>[18x]MTAVSEFRPGLEGVPATLSSISFVDGQRGVLEYRGISIEQLAQQSSFLETAYLLIWGHLPTQQELTEFEHEIRYHRRIKFRIRDMMKCFPDSGHPMDALQASAAALGLFYSRRALDDPEYIRAAVVRLLAKIPTMVAAFQLIRKGNDPIQPRDELDYAANFLYMLTEREPDPVAARIFDICLTLHAEHTINASTFSAMVTASTLTDPYAVVASAVGTLAGPLHGGANEEVLDMLEAIGSVENVEPYLDHCIATKTRIMGFGHRVYKVKDPRAVILQNLAEQLFDIFGHDPYYEIAVAVEKAAAERLSHKGIYPNVDFYSGLVYRKLGIPSDLFTPVFAIARVAGWLAHWKEQLNENRIFRPTQIYTGSHNLDYTPIADRDLAIESDLEHHHHHH

Here we report the discovery of a natural protein, citrate synthase from the cyanobacterium Synechococcus elongatus, which self-assembles into Sierpiński triangles. Bacterial citrate synthase (CS) proteins are homo-oligomeric enzymes that can assemble into dimers and hexamers. CS catalyses the condensation of acetyl-CoA and oxaloacetate to citrate as the first step in the tricarboxylic acid cycle. Using cryo-electron microscopy, we reveal how the fractal assembles from a hexameric building block.

Three dimers are first arranged in a hexameric ring and three hexamers then connect into a triangle. In the 18mer (level 1), CS dimers assemble into hexamers through a heterologous interface similar to known hexameric CS proteins. The 18mer is then formed through an additional contact between two dimers of adjacent hexamers. This interface has an unusual geometry, whereby only one monomer from each dimer participates in the interaction. The two participating monomers form an interface between the amino terminus of one monomer and the carboxy terminus of the other and vice versa. An interaction between the residue E6 from one monomer and H369 of the other establishes an important contact, and mutating either E6 or H369 to alanine or deleting amino acids 2–6 (Δ2–6 SeCS) abolishes the formation of fractals. In the two non-participating monomers, the termini face outwards. They cannot engage in the same interaction with another dimer without causing a steric clash and thereby passivate the edge of the triangular assembly. In the 18mer, the non-equivalence between chains allows the interaction to form at the correct angle and ensures that no more dimers can associate into it.>MGNVQTSVNTYNITGDGNSFTPTSDMTSTAAPAIDLKPGVLN[10x];>[10x]PTGKLWRPVGTSVATIDSLAIVSDRFGQYSFVNEGMRETFSKALFDINMWQPLFQATKTGCGPIVLSSFTTTTSGYVGATAGDALDNPVTNGVFISTVQIMNLQRTIAARMRDVALWQKHLDTAMTMLTPDISAGSASCNWKSLLAFAKDILPLDNLCLTYPNEFYNVAIHRYPALKPGNPDTKLPDAQAHPLGEVAGAFNAATSEVGSLVGSSSTLSQAISTMAGKDLDLIEADTPLPVSVFTPSLAPRSYRPAFIKPEDAKWIAEFNNSSLIRKTLTYSGATYTVQLGPGPTRVIDMNAMIDSVLTLDVSGTILPYDTNPDLSTSVPAFVLIQTSVPIQQVTTAANITAITVVSAAGASAINLAINVRGQPRFNMLHLQATFERETITGIPYIYGLGTFLIPSPTSSSNFSNPTLMDGLLTVTPVLLRETTYKGEVVDAIVPATVMANQTSEEVASALANDAIVLVSNHLNKLANVVGDAIPVASRTDDSATSAIVSRLAVQHKLSQVGQASPTPPDYPLLWRRAKRAASMFVSNPSLALQVGIPVLTQSGMLSALTSGVGTALRTGSLGKGVTDASEKLRARQSLTVAKQAFFDQIGSLWPGK;>[2x]MAQRQFFGLTYNFYGQPAPLFDLNDLQELAGCYARPWTSRFSHLAISTGSLPVWSARYPSVASRNIVVNTLLGAHLNPFAGGQITSHQGITWRDPVLSSLAPVPAIQPPPVWAVAENVLLDSNNYPTYVLNLSSMWPINQDVHIMTMWALSDQGPIYHLEVPVDPMPAATTAALMAYTGVPIAHLAQTAYRFAGQLPQSPDSTMVSTIRWLSAIWFGSLTGRLNRSRTCNGFYFEFAKPALNPDQAVLKWNDGARAAPPAAAQSSYIRCISPHWQHQIVEVAGALMSQSVTAVTGLPALIDEATLPAWSQGVANLTGNGQGVVPCLDYNPVPMAAARHLQWRQDGLITAAQEAQLNNDYTAYALTIERHLTAMLVANPIAAGRMPIQPFNAADFGQAGQTAAAVALAQAMFV;> MAAVFGIQLVPKLNTSTTRRTFLPLRFDLLLDRLQSTNLHGVLYRALDFNPVDRSATVIQTYPPLNAWSPHHAFIENPLDYRDWTEFIHDRALAFVGVLTQRYPLTQNAQRYTNPLVLGAAFGDFLNARSIDIFLDRLFYDPTQDSPITAITKFPYQWTIDSNVTTDSVRTSAGCKYITLYGYDPSRPSTPATYGKHRPTYATVFYYSTLPARSRLLANLAAGPTVLEHFDSPTYGPHLLLPQTGDVLGYSSSLISQAALLMVESVMDALRDNANASASTAVTRLDQSYHPVTSFDPSTFNTLLQRATNLALLAVQGVQSESAIPAIPTMSDVRSFVARLMAEGDPQQWFPYRVDQILYWPESPFVPPIGPFYAPFRPVNFPFTTGSYTVVPDASRPLRLLPQYRNATITVQQADDAYEDTALSPLITTHGFCVTGGVFTSIYDISGDPTAYPPAQLVDAPNDYFDRERMARRDLFRRLRAPADRSAIKDRAVFDFLASLVNPTTANPVLDTSFSMAYLGASSAHANADEPVILADIRSGSIPGLPIPRRIVQFGYDVVHGSLLDLSRAVPTGTFGLVYADLDQVEDAGTDMPAANRAAIAMLGTALQMTTAGGVSVLKVNFPTRAFWTQVFNLYATHATTLHLVKPTIVNSSEVFLVFGGRQSNGALRSTTALQRALLSLYARNAAIDRAVTHIPFFGVPDDGTSDLGIDAVRLFDPMFSDAVANLPSNALASLVSRVVPSSIMFTRVPSNGPVSTTIYGKRTFLSNRRRARLRDVPMLITTTLVHQRRFTTPPTFTLFSSEAVPVTTLVAAGYNSFISEQTRNPNLAHLLDLGTGPECRILSLIPPTLQVTMSDSRPCAELMASFDPALTAYVQGDYSTAAFWNGIRCDSATAIFTIGAAAAAAGTDLIAFVQQLIPRIVAAGGTRMWLQLNTPLYEVSSLPDLIEIDLRDHVYRFNGGERVEPYADPVPLQQAIAALLPAAALSWHTLSPTCDWLPYIIGVGSPLNLSDINTAISYSRLTPILHIDTTTPPLRVNPVPTPLNQQCAIRITSLDPAAVLSVQHNGVEVIGGTPGNVISVAGAAALQYILANQEFLLQFTPTLPGIFDVFLTTLGQPPVPRGSFTITPPPTTVALNMPPPRQLDFTDVGNDARITCDPYYQLAVCIFKDGQYVRVNPEKASVVTNAPNRDLHFVLDLADNHVLLYLCDVTPSGLGDRIAFPIVDIYRIAFPRNTPVRASLPYTGGGAHLTSGGNPFMSLTTPPAVLPAGVALAALSTSVATQYPTYTLPAGVYEYVIE;>[2x]MPRRSARKAQSAIASPADTNVVPAKDAPTTNSPPSTTS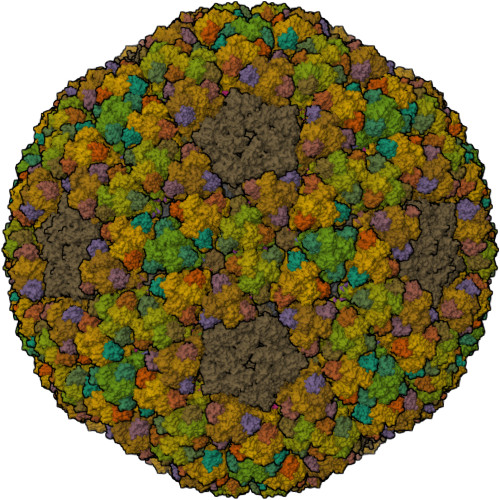PNQAAADANQQQAGIVSSQSGPNAVGDSAPSSSVNNDGDIITRPTSDSIAAVANATKPAAVVSDPQSMKVTPIVNPSSYVCNVCNARFSTMSALSEHLRSDHRDDASTLLATPMINNAIRSFLTAWDDIRILSPDVSSKSLSAYLDSAVANGPELIIEDTGLCTSFMLLDNIPSAHLTKELIGFTWFMQMYQMTPPLPEGAVNRIVCMTNWASLGDEGRGLEVRLPPPTDSSVHAYKTVLSRGYIDNAQFNPLALRSNVLLMLLQFTLSNLKINKSSTFTSDVTTITSGRMIRAFEGRPELLALAYPGRAVLPTQTKNAQFLSTAIADRIGRLDRANLIGGEVSAMVECMELCDALTLHIRETYIMLLRSMHQDPTQIVQIVNECANNLLNSTIPISLRPTILCPWFASSEDLRLQQVMHLVNISSNTAAALPLVEALSTLLRSVTPLVLDPTVLTNAITTISESTTQTISPISEILRLLQPMGNDYAAFWKCIASWAYNGLVTTVLSEDAFPDSSQSITHLPSMWKCLFLTLAGPMTSDPHSPVKVFMALANLLAQPEPIAIGVPGMHQTTPASQFSHPGVWPPGFLNPQLINPQQAPLLRAFAEHIRANWPQPSEFGYGSTLQGSANLFIPSNRMVYPWPNQPLPRLTVAPTYDSAMSNWISTTIAFFIRVVNSVNMTATVNDLTRRTMTGVMTAMRQVKTMTPFYIQHMCPTELSVLASVTVTPPFQVPFTRLVQNDVITNVLVARVDPAQRGDAAVDIRATHATFAAALPVDPAAIVVAMLCGQTETNLIPSHHYGKAFAPLFASNAMFTRNQRAVITREAFVCARSAVAQCQDAGFLVPRPLDALRQFDVTSAAAAEIMHAVNDAFKTAFDLDGALLDGLALYGDPRIADLSAAYLQYGGNVVREHVPPGPSHIHRALQQVESTFMAEMNLFNVARGNLYLVQTATNGNWSPMAPVAAPPFVRGGPNVRVVGRFGTIVPRPNGLEPQLIDDGNVPRDIAGDWVYPSDVLQVSVAVFRDYVWPMVKAGRTRVLVELGHYVYTLHYYDPQISLDEAPILEEWLSKINPAGIPPVPFCIPIPQVYPCITARRVHYAFTSENNNDSLFSTNAASIDTAFGENAAVSPLRWPGLVDPNYRVGTNDLPNRITLYNSLYRYNFTYPTLDGIMYVRSAT;>[10x]MPLHMIPQVAHAMVRAAAAGRLTLYTRTRTETTNFDHAEYVTCGRYTICAFCLTTLAPHANVKTIQDSHACSRQPNEAIRSLVEVSDKAQTALVGSRTVDYHELDVKAGFVAPTADETIAPSKDIVELPFRTCDLDDSSATACVRNHCQAGHDGVIHLPILSGDFKLPNEHPTKPLDDTHPHDKVLTRCPKTGLLLVHDTHAHATAVVATAATRAILMHDLLTSANADDGHQARSACYGPAFNNLTFACHSTCASDMAHFDCGQIVGLDLHVEPSD>SKEGSVAPKERINIKYIPATGDAQAEVELPLKTLVVGDFKGHAEQTPLEERATVTVDKNNFEAVMRESELKITATVKNKLTDDENAELPVELNFKSLADFAPDAVASQVPELKKLIELREALVAL[30x];>NKSLVDQMLVELDKKISAQMDEILHNSQFQAMESAWRGLKLFVDRTDFRENNKVEILHVTKDELLEDFEFAPETAQSGLYKHVYSAGYGQFGGEPVGAIIGNYAFTPSTPDMKLLQYMGALGAMAHAPFISSVGPEFFGIDSFEELPNIKDLKSTFESPKYTKWRSLRESEDARYLGLTAPRFLLRVPYDPIENPVKSFNYAENVSASHEHYLWGNTAFAFATRLTDSFAKYRWCPNIIGPQSGGAVEDLPVHVFESMGALQSKIPTEVLITDRKEFELAEEGFIALTMRKGSDNAAFFSANSIQKPKVFPNTKEGKEAETNYKLGTQLPYMMIINRLAHYVKVLQREQIGAWKERQDLERELNSWIKQYVADQENPPADVRSRRP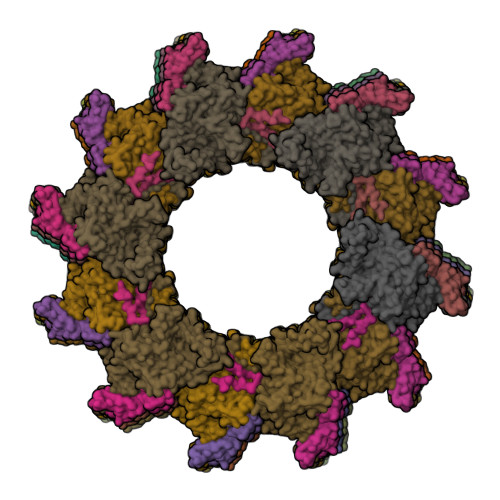LRAARIEVMDVEGNPGWYQVSLSVRPHFKYMGANFELSLVGRLDQA[30x]Cell surface layers (S-layers) form symmetrical lattices on many bacterial and archaeal cells, playing essential roles such as facilitating cell adhesion, evading the immune system, and protecting against environmental stress. The S-layer is built from one or more (glyco)-protein subunits, S-layer proteins (SLPs), that self-assemble into a highly flexible and dynamic lattice through an entropy-driven process, allowing for structural adaptation in response to changing environmental conditions. In this study, we introduce the SymProFold pipeline, which utilizes the high accuracy of AlphaFold-Multimer predictions to derive symmetrical assemblies from protein sequences, specifically focusing on two-dimensional S-layer arrays and spherical viral capsids. The predicted models were validated using available experimental data at the cellular level, and additional crystal structures were obtained to confirm the symmetry and interfaces of several SymProFold assemblies.

High-resolution experimental data confirming the proposed assemblies at the atomic level is very scarce. Based on our predicted models of Viridibacillus arvi and Methanococcus voltae, we designed constructs (see Methods section) containing only the domain responsible for the formation of either the 4-fold or 2-fold axis. H Proposed assembly of Methanococcus voltae (gray) with the 2-fold symmetry axis of the anchoring region is shown in orange. Aligning the crystal structures with the SymProFold models revealed a great similarity, with RMSD values of 0.65 Å for V. arvi and 1.38 Å for M. voltae, further confirming our predicted assemblies. The SymProFold prediction of S-layers from P. abyssi, M. voltae, T. camini, T. thioreducens, and M. vannielii, even though different in sequence, size, and domain structure, show an analog domain arrangement as the crystal structure of M. acetivorans SLP and reveal a dimeric anchor, which has not been described previously. For S-layers from Vibrio aerogenes, Paenibacillus naphtalenovorans, Pyrococcus abyssi, Methanococcus voltae, Thermococcus camini, Thermococcus thioreducens, and Phocaeicola vulgatus, no experimental data on the unit cell parameters, structure, or symmetry are reported.

> MVEKIGDVEGFKVIDNGEPTADIVVGSTAAAADVVSAANVAAKVGSMMFKEGEGGSDAKAPVAFKAPLAVLDTEVSLDAANKKLILVGGPVANALTKELADAGKIEMTVESPATLAVVAGAANGNDVLVVAGGDRAATAEAANALIEMLLEHHHHHH>GPLGSMATTNDSAVLFYIVASQKKLSFDYTPNWGRGSP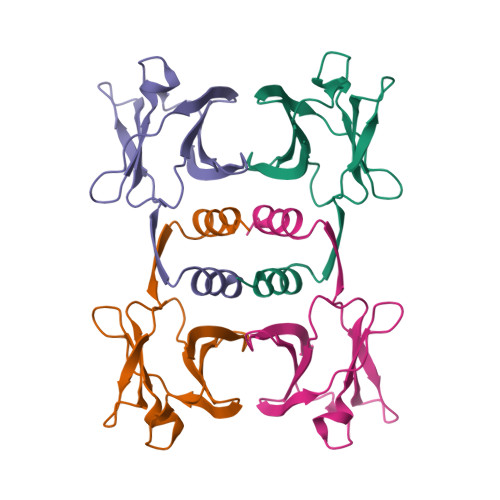NSYIDNLTFPRVLTNKPYKYRVVKAGQDLGVRDSYSVQSDGSQKVNFLEYNAGRGIADTQTIQVYVVDPDNGNQYLVAQWKHHHHHH[8x]> AAPTAYTPLDVAQAYQFPEGLDGQGQCIAIIELGGGYDETSLAQYFAS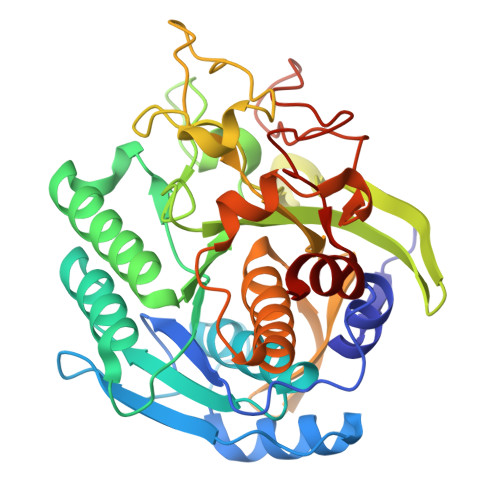LGVSAPQVVSVSVDGATNQPTGDPNGPDGEVELDIEVAGALAPGAKIAVYFAPNTDAGFLNAITTAVHDPTHKPSIVSISWGGPEDSWAPASIAAMNRAFLDAAALGVTVLAAAGDSGSTDGEQDGLYHVDFPAASPYVLACGGTRLVASAGRIERETVWNDGPDGGSTGGGVSRIFPLPSWQERANVPPSANPGAGSGRGVPDVAGNADPATGYEVVIDGETTVIGGTSAVAPLFAALVARINQKLGKPVGYLNPTLYQLPPEVFHDITEGNNDIANRARIYQAGPGWDPCTGLGSPIGIRLLQALLP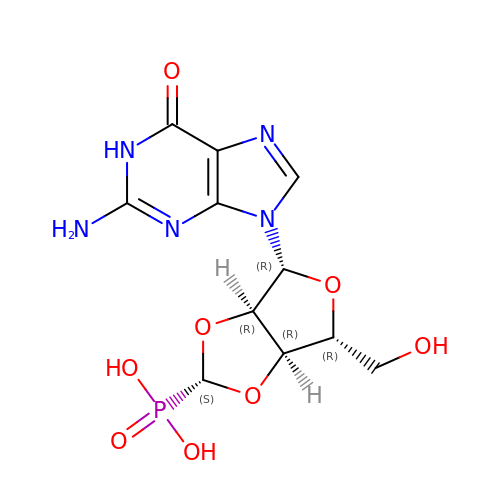(2S,4R,6R,6AS)-4-(2-AMINO-6-OXO-1,6-DIHYDROPURIN-9-YL)-6-(HYDROXYMETHYL)-TETRAHYDROFURO[3,4-D][1,3]DIOXOL-2-YLPHOSPHONIC ACID | C11 H14 N5 O8 P | GKAPYWCOOQBBHV-KXSYMAMXSA-N>SNAMLRRLFKKKYVCVRQYDLTDCGAACLSSIAQYYGLKMSLAKIREMTGTDTQGTNAYGLIHAAKQLGFSAKGVKASKEDLLKDFRLPAIANVIVDNRLAHFVVIYSIKNRIITVADPGKGIVRYSMDDFCSIWTGGLVLLEPGEAFQKGDYTQNMMVKFAGFLKPLKKTVLCIFLASLLYTALGIAGSFYIKFLFDDLIKFEKLNDLHIISAGFAVIFLLQIFLNYYRSILVTKLGMSIDKSIMMEYYSHVLKLPMNFFNSRKVGEIISRFMDASKIRQAISGATLTIMIDTIMAVIGGILLYIQNSSLFFISFIIILLYGIIVTVFNKPIQNANRQIMEDNAKLTSALVESVKGIETIKSFGAEEQTEKSTRDKIETVMKSSFKEGMLYINLSSLTGIVAGLGGIVILWAGAYNVIKGNMSGGQLLAFNALLAYFLTPVKNLIDLQPLIQTAVVASNRLGEILELATEKELREDSDDFVISLKGDIEFRNVDFRYGLRKPVLKNINLTIPKGKTVAIVGESGSGKTTLAKLLMNFYSPEKGDILINGHSIKNISLELIRKKIAFVSQDVFIFSGTVKENLCLGNENVDMDEIIKAAKMANAHDFIEKLPLKYDTFLNESGANLSEGQKQRLAIARALLKKPDILILDEATSNLDSITENHIKDAIYGLEDDVTVIIIAHRLSTIVNCDKIYLLKDGEIVESGSHTELIALKGCYFKMWKQTENTLA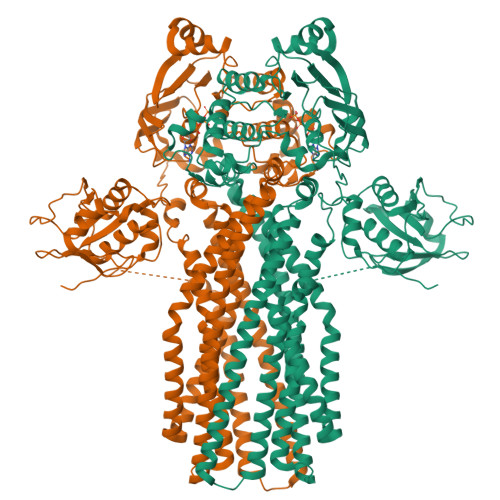S[2x]> VDCSEYPK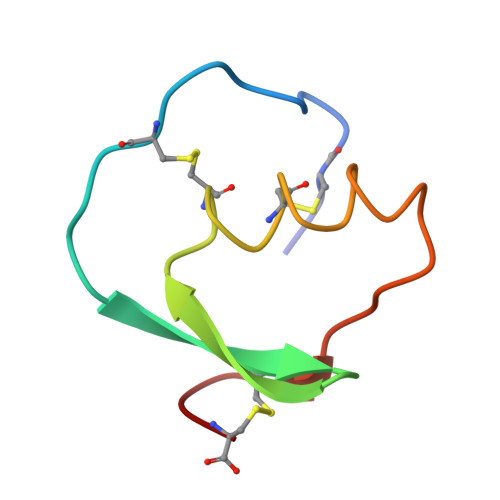PACTYEYRPLCGSDNKTYGNKCNFCNAVVESNGTLTLSHFGKC>MGRAHKETLDKLTNAAINKINLLNTSKVKYLVSSAFAGLYVGIGILLIFTIGGLLTDAGSPMTKIVMGLSFAIALSLVIMTGTELFTGNNMVMSAGMLNKGVSIKDTSKIWAYSWVGNLIGALVLGIIFVGTGLVDKGPVAEFFANTAASKASMPFTALFFRGILCNILVCVSVLCSFRTNSDTAKIIM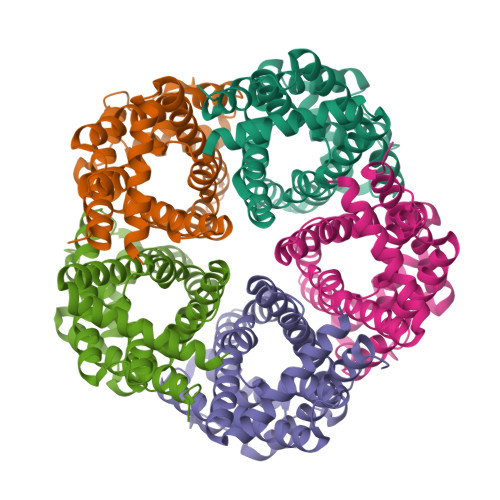IFLCLFAFITSGFEHSVANMTIYSVSLFSPTISTVTIGGAIYNLVAVTLGNIVGGALFMGLGTYILGKEKLNAAAENLY[10x]(4P)-4-[6-fluoro-5-(2-methoxyanilino)-1H-indazol-1-yl]-N-(oxetan-3-yl)thiophene-2-carboxamide | 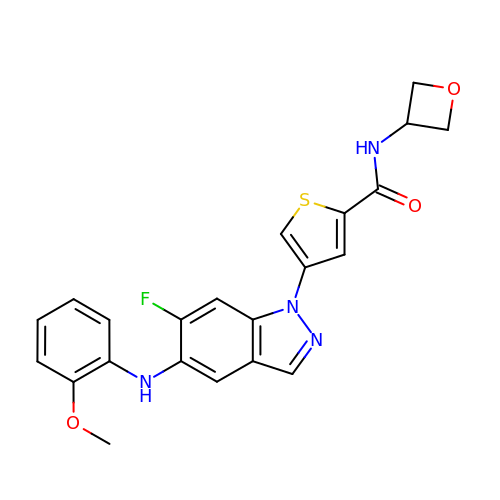C22 H19 F N4 O3 S | GYCODKDGFRRIIQ-UHFFFAOYSA-N> MGSVTPIPLPKIDEPEEYNTNYILFWNHVGLELNRVTHTVGGPLTGPPLSARALGMLHLAIHDAYFSICPPTDFTTFLSPDTENAAYRLPSPNGANDARQAVAGAALKMLSSLYMKPVEQPNPNPGANISDNAYAQLGLVLDRSV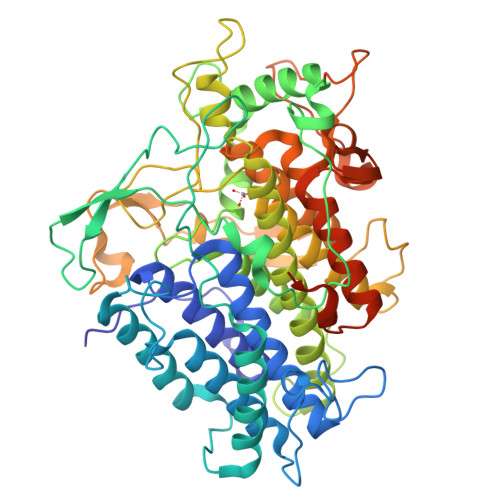LEAPGGVDRESASFMFGEDVADVFFALLNDPRGASQEGYHPTPGRYKFDDEPTHPVVLIPVDPNNPNGPKMPFRQYHAPFYGKTTKRFATQSEHFLADPPGLRSNADETAEYDDAVRVAIAMGGAQALNSTKRSPWQTAQGLYWAYDGSNLIGTPPRFYNQIVRRIAVTYKKEEDLANSEVNNADFARLFALVDVACTDAGIFSWKEKWEFEFWRPLSGVRDDGRPDHGDPFWLTLGAPATNTNDIPFKPPFPAYPSGHATFGGAVFQMVRRYYNGRVGTWKDDEPDNIAIDMMISEELNGVNRDLRQPYDPTAPIEDQPGIVRTRIVRHFDSAWELMFENAISRIFLGVHWRFDAAAARDILIPTTTKDVYAVDNNGATVFQNVEDIRYTTRGTREDEEGLFPIGGVPLGIEIADEIFNNGLKPTPPEIQPMPQETPVQKPVGQQPVKGMWEEEQAPVVKEAP> MTCNFETADRRKRFWTTQVAACGQSSDDCGDCARPGLQLLCNGEGRITIATDNYVAGLALNILLTDASKADTGCGWTPGNRGGFWGDSFRSDNMRSGSKIRQVTARGSMRETVALIRAYAIDDLKKLVAYGVAKSVDVDLTYQGSNKIDMTIMIQGVDGNESRVGLTGERIANA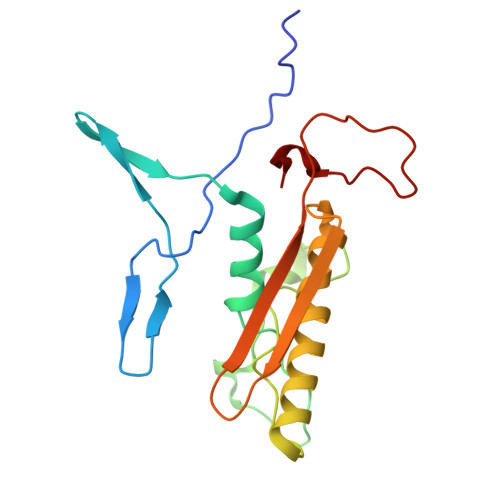WVWS ICV, however, has only one major surface glycoprotein, the hemagglutinin-esterase-fusion (HEF) protein, which possesses all-in-one of receptor binding, receptor destroying and membrane fusion activities. To further evaluate the infectivity and transmissibility of IDV, we expressed and purified the ectodomain of D/OK HEF, and determined that it also uses 9-O-Acetyl-Sia as its receptor by glycan microarray. We also solved the crystal structure of D/OK HEF, both in its native state (resolution of 2.4 Å) and in complex with its receptor analogue (resolution of 3.1 Å), and the structure of the enzymatically inactive HEF (resolution of 2.4 Å) alone and in complex with two receptor analogs respectively (both resolutions of 2.2 Å). Indeed, our results show that IDV HEF is functionally and structurally similar to ICV HEF, but with some distinct characteristics.

To avoid the enzymatic cleavage of the receptor substrates, we generated the catalytic mutant for the binding experiments and for the structures of the relevant complexes. Thus, we designed the enzymatically inactive HEF protein (HEF-mut) containing S57A, D356A and H359A substitutions, and expressed it using the same method as wild type protein. For the IDV HEF-mut/receptor complex structures, interpretable electron density is observed for all the three glycan rings of 9-O-Ac-3'SleC, including Neu5,9Ac2 (9-O-Ac-Sia-1), galactose-2 (Gal-2), and N-acetylglucosamine-3 (GlcNAc-3); while for 9-O-Ac-3'SLN, electron density for the first two sugars is well defined. But the majority of the interactions between ligands and IDV HEF are made by the 9-O-Ac-Sia-1 moiety, whereas the glycan portion of the ligands do not make significant contacts with IDV HEF, except for a hydrogen bond between the Gal-2 of 9-O-Ac-3'SLN and S173. Compared with the ICV HEF receptor complex, the 9-O-Ac-Sia-1 of the receptor bound to IDV HEF displays a very similar orientation. The 9-O-acetyl group of the receptor docks into a nonpolar, hydrophobic pocket, formed by V275, F229, F240 and F297. The acetyl carbonyl oxygen forms a hydrogen bond with the hydroxyl group of Y231 (ICV HEF: Y227). The 5-N-acetyl group of the ligand fits into a hydrophobic pocket formed mainly by W185, and forms a hydrogen-bonding interaction with A172. In addition, the carboxyl group of C1 formed two hydrogen-bonding interactions with S173.

>ELICIVQRVNESFSLHSGFGGNVYSMKTEPMTGFTNVTKGASVINQKDWIGFGDARTDLTNDQFPASSDVPLAVAKKFRSLSGASLMLSAFGPPGKVDYLYQGCGKEKVFYEGVNWSPEAGIDCFGSNWTQTKKDFYSRIYEAARSSTCMTLVNSLDTKISSTTATAGTASSCSSSWMKSPLWYAESSVNPGAKPQVCGTEQSATFTLPTSFGIYKCNKHVVQLCYFVYENKAKFNTFGCGDYYQNYYDGNGNLIGGMDNRVAAYRGIANAGVKIECPSKILNPGTYSIKSTPRFLLVPKRSYCFDTDGGYPIQVVQSEWSASRRSDNATEEACLQTEGCIFIKKTTPYVGEAADNAGDIEMRQLLSGLGNNDTVCVSQSGYTKGETPFVKDYLSPPKYGRCQLKTDSGRIPTLPSGLIIPQAGTDS[2x];>[2x]IFGIDDLIFGLLFVGFVAGGVAGGYFWGRSNGGGGGASVSSTQAGFDKIGKDIQQLRNDTNAAIEGFNGRIAHDEQAIKNLAKEIEDARAEALVGELGIIRSLIVANISMNLKESLYELANQITKRGGGIAQEAGPGCWYVDSENCDASCKEYIFNFNGSATVPTL2-amino-6-[(1Z)-1,2-dihydroxyprop-1-en-1-yl]-7,8-dihydropteridin-4(3H)-one 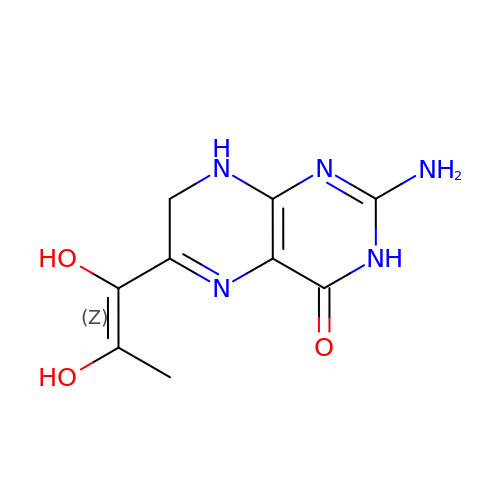| C9 H11 N5 O3 | FYDGMRRMOMSOLR-UTCJRWHESA-N>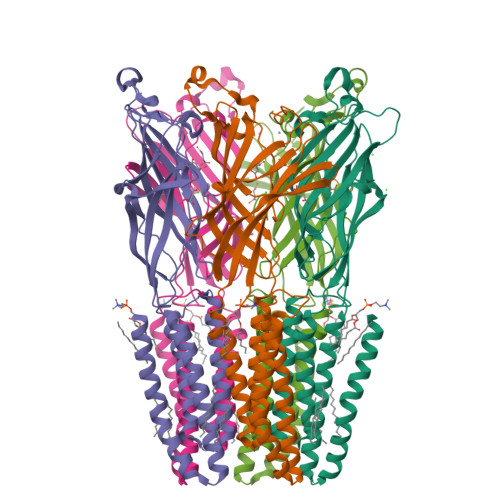[10x]GQDMVSPPPPIADEPLTVNTGIYLIECYSLDDKAETFKVNAFLSLSWKDRRLAFDPVRSGVRVKTYEPEAIWIPEIRFVNVENARDADVVDISVSPDGTVQYLERFSARVLSPLDFRRYPFDSQTLHIYLIVRSVDTRNIVLAVDLEKVGKNDDVFLTGWDIESFTAVVKPANFALEDRLESKLDYQLRISRQYFSYIPNIILPMLFILFISWTAFWSTSYEANVTLVVSTLIAHIAFNILVETNLPKTPYMTYTGAIIFMIYLFYFVAVIEVTVQHYLKVESQPARAASITRASRIAFPVVFLLANIILAFLFFGF>[2x]MRLFLSLPVLVVVLSIV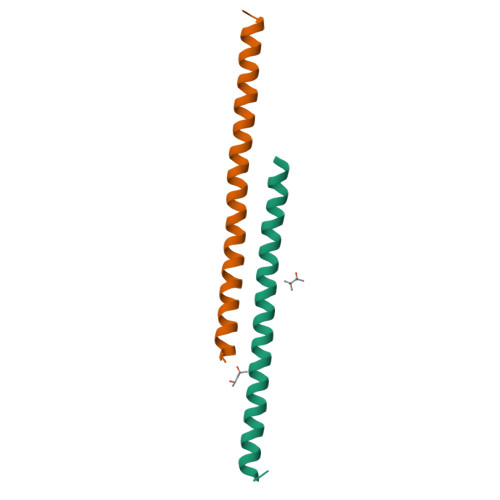LEGPAPAQGTPDVSSALDKLKEFGNTLEDKARELISRIKQSELSAKMREWFSETFQKVKEKLKIDS> ICATA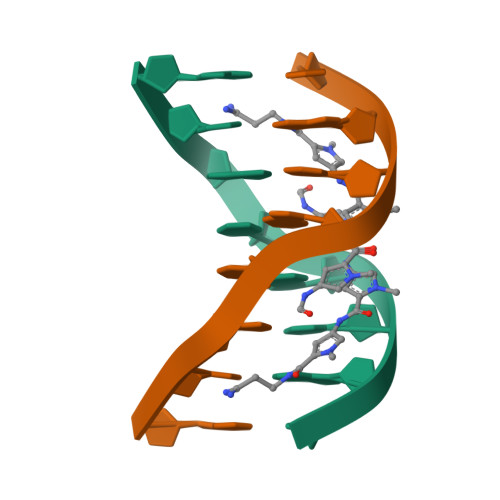TIC>MILVTGSSGQIGTELVPYLAEKYGKKNVIASDIVQRDTGGIKFITLDVSNRDEIDRAVEKYSIDAIFHLAGILSAKGEKDPALAYKVNMNGTYNILEAAKQHRVEKVVIPSTIGVFGPETPKNKVPSITITRPRTMYGVTKIAAELLGQYYYEKFGLDVRSLRYPGIISYKAEPTAGTTDYAVEIFYYAVKREKYKCYLAPNRALPMMYMPDALKALVDLYEADRDKLVLRNGYNVTAYTFTPSELYSKIKERIP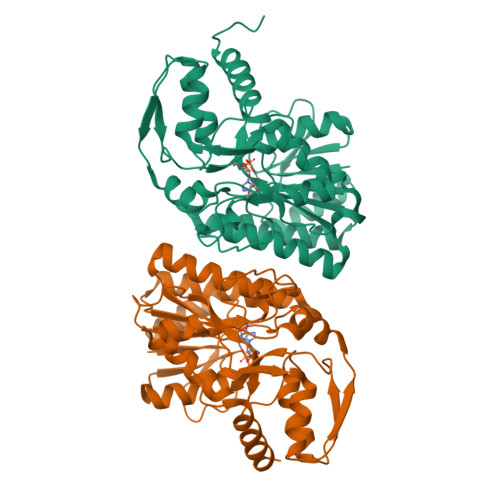EFEIEYKEDFRDKIAATWPESLDSSEASNEWGFSIEYDLDRTIDDMIDHISEKLGIEGKHAL[2x]> MHELIKYQFNTRRKKYGTGAALSLLNGNVGHEVLAFHKKLPNYAVTPLHNLAHLSQRLGLGSIHIKDESWRFGLNAFKGLGGSYAVGKYLADKLQCDINSLSFAALNTPEIKEKIKDCVFVTATDGNHGRGVAWAAEQLGLKAVVYMPKGSSLIRAENIRHHGAECTITDLNYDDAVRLAHRMAQTKGWVLLQDTAWTGYEEIPTWIMQGYMTLAVEAYEQLAE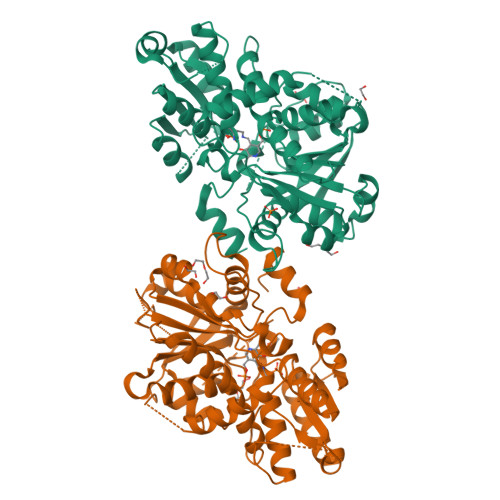TNSPLPTHLILQAGVGSFAGSVMGYFVEKMQENIPNIIVVEPHQANCLYQSAVMDDGQPHCVTGDMATIMAGLACGEPNIISWPIIRDNTSCFISADDCLAAKGMRISAAPRPGTDTPFISGESGAIGVGLLYELMNNMHYQDLANRLQLDASAHVLLISTEGDTSPDIYEDIVWNGRSA;>[3x]MHELIKYQFNTRRKKYGTGAALSLLNGNVGHEVLAFHKKLPNYAVTPLHNLAHLSQRLGLGSIHIKDESWRFGLNAFKGLGGSYAVGKYLADKLQCDINSLSFAALNTPEIKEKIKDCVFVTATDGNHGRGVAWAAEQLGLKAVVYMPKGSSLIRAENIRHHGAECTITDLNYDDAVRLAHRMAQTKGWVLLQDTAWTGYEEIPTWIMQGYMTLAVEAYEQLAETNSPLPTHLILQAGVGSFAGSVMGYFVEKMQENIPNIIVVEPHQANCLYQSAVMDDGQPHCVTGDMATIMAGLACGEPNIISWPIIRDNTSCFISADDCLAAKGMRISAAPRPGTDTPFISGESGAIGVGLLYELMNNMHYQDLANRLQLDASAHVLLISTEGDTSPDIYEDIVWNGRSALEHHHHHH>PLGSMVFERFTERAIRAIIFSQKEAKSLGKDMVYTQHLLLGLIAEDRDPQGFLGSGITIDKAREAVWSIWDEANSDSKQEEASSTSYSKSTDMPFSISTKRVFEAAVEYSRTMDCQYIAPEHIAVGLFTVDDGSAGRVLKRLGANMNLLTAAALTRLKGE[2x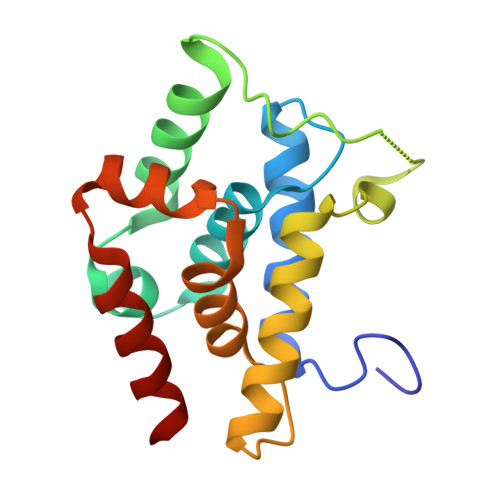]>[11x]MSLQGIHLSDLSYKHAILKESQYTIKRDVGTTTAVTPSSLQQEITLLCGEILYAKHADYKYAAEIGIQYISTALGSERVQQILRNSGSEVQVVLTRTYSLGKIKNNKGEDLQMLDIHGVEKSWVEEIDKEARKTMATLLKESSGNIPQNQRPSAPDTPIILLCVGALIFTKLASTIEVGLETTVRRANRVLSDALKRYPRMDIPKIARSFYDLFEQKVYHRSLFIEYGKALGSSSTGSKAESLFVNIFMQAYGAGQTMLRWGVIARSSNNIMLGHVSVQAELKQVTEVYDLVREMGPESGLLHLRQSPKAGLLSLANCPNFASVVLGNASGLGIIGMYRGRVPNTELFSAAESYAKSLKESNKINFSSLGLTDEEKEAAEHFLNVSDDSQNDYEKHHHHHH;>EDDIYQLIM[11x]

The viral genome is encapsidated in a sheath of oligomerized copies of the nucleoprotein N, forming a ribonucleoprotein complex termed nucleocapsid. The nucleocapsid is the template for transcription and replication by L, which is also dependent on the obligate polymerase cofactor, the phosphoprotein P, together forming the active L/P holoenzyme. In oligomerized and RNA-bound N (N-RNA) the nucleic acid is threaded along an extended groove in between the NTDs and CTDs of laterally connected N protomers. An important function of the C-terminal domain of P in nsNSVs is to bind to assembled N-RNA, forming an N-RNA/P complex.

We incubated N-RNA preparations with a ~ 100-fold molar excess of synthetic peptide covering the 9 last residues of PCT (N-EDDIYQLIM-C). Cryo-EM analysis of the N-RNA/P complex revealed the presence of the same classes of assemblies as was the case with the apo sample. We carried out 3D reconstruction of 10-mers, 11-mers, and spiral particles of the N-RNA with PCT. In the case of the spiral particle, we restricted ourselves to rigid-body placement of N-RNA/P protomers due to mediocre map quality, as before with N-RNA. Lastly, viewed in the context of an N-RNA assembly, the PCT binding site is located such that P attaches to a region of the nucleocapsid that protrudes at a far radius from the helical axis. This may facilitate accessibility to P-binding, even in light of the conformational heterogeneity of the nucleocapsid.> ANSTAELEELLMQRSLTDPQLQAAAAAAADFRILPDATVISIGGQSVIDRGRAAVYPLVDEIVAARKNHKLLIGTGAGTRARHLYSIAAGLGLPAGVLAQLGSSVADQNAAMLGQLLAKHGIPVVGGAGLSAVPLSLAEVNAVVFSGMPPYKLWMRPAAEGVIPPYRTDAGCFLLAEQFGCKQMIFVKDEDGLYTANPKTSKDATFIPRISVDEMKAKGLHDSILEFPVLDLLQSAQHVR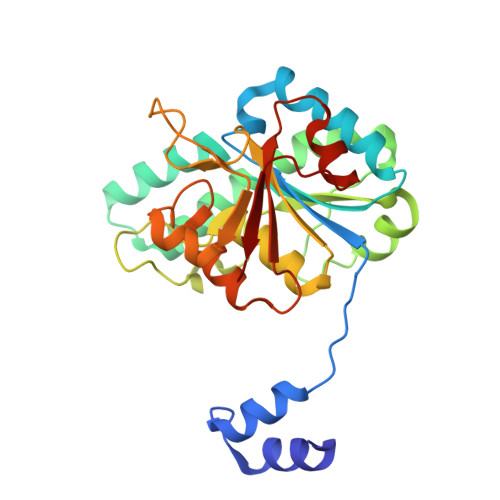EVQVVNGLVPGNLTRALAGEHVGTIITAS> TNFDAERDALNIETAIKTKGVDEVTIVNILTNRSNAQRQDIAFAYQRRTKKELASALKSALSGHLETVILGLLKTPAQYDASELKAS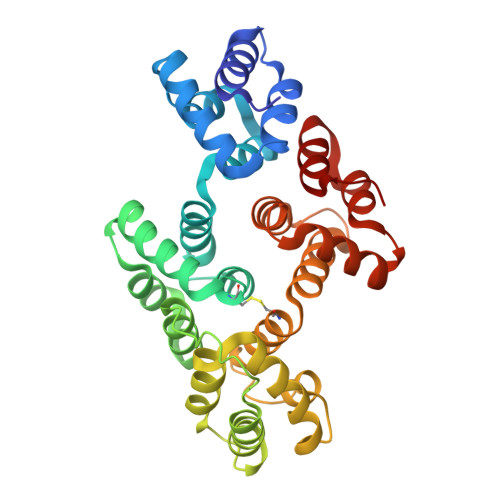MKGLGTDEDSLIEIICSRTNQELQEINRVYKEMYKTDLEKDIISDTSGDFRKLMVALAKGRRAEDGSVIDYELIDQDARDLYDAGVKRKGTDVPKWISIMTERSVPHLQKVFDRYKSYSPYDMLESIRKEVKGDLENAFLNLVQCIQNKPLYFADRLYDSMKGKGTRDKVLIRIMVSRSEVDMLKIRSEFKRKYGKSLYYYIQQDTKGDYQKALLYLCGGDD>MAFQLHPRLQQDCIVLGNLPLCKVLLIKEDIGPWLILVPRIEELKEIHHMTDEQQIQFIKESSAVA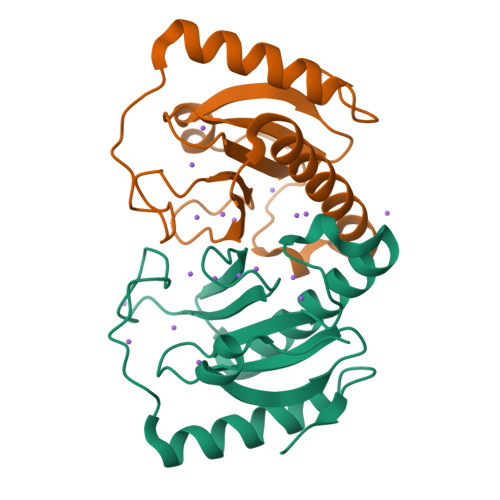QLLEDNFSPDKINIGALGNLVPQLHIHHIARFTTDVAWPGPVWGNTTGVIRAQSSQTQLVDLLRDKLSNISGFKRLEHHHHHH[2x]> GSTYDALRRQLIPSFDLLYGSAVSVVAMSVPATARILDLGAGTGLLGAALRERLPDAELLLQDRSQAMLEQARQRFADDDQVAIRVADHLDELPAGPFDAVVSALSIHHLEHQDKQDLFTRIRKILRPGGIFVNVEQVLAPTSELEKMYDRQHEAHVLASDTPAEEWAAGRERMKHNIPIDVETQIQWLRDAGFTTADCLAKDWRFATYAGWNGS

Here, we characterize the O-methyltransferases BelI and CysG, which catalyze the initial step of β-lactone formation. Employing techniques such as crystallography, computational analysis, mutagenesis, and activity assays, we identified a His-His-Asp (HHD) motif in the active sites of the two enzymes, which is crucial for binding a catalytically active calcium ion. As expected, BelI as well as CysGΔN16 adopt the class I methyltransferase Rossmann fold, characterized by a core domain of a seven-stranded β-sheet flanked by α-helices. The HHD-motif enables regiospecific C1-carboxy group methylation of their respective malic substrates.

Due to the high crystallization tendency of CysGΔN16, subsequent mutagenesis experiments were focused on this variant. This approach enabled the production of both full-length and N-terminal truncated mutants in high purity, which were characterized in activity assays and used for structural studies. Conservative asparagine replacements in the HHD motif resulted in CysG variants that remained active. CysGfl-D191N showed a 56% decrease in substrate turnover, while CysGfl-H122N and CysGfl-H123N were fully active compared to wt but were inactivated with EDTA.>GSHMIKVLSPAKINLGLWVLGRLPSGYHEILTLYQEIPFYDEIYIREGVLRVETNIGIPQEENLVYKGLREFERITGIEINYSIFIQKNIPPGAGLGGGSSNLAVVLKKVNELLGSPLSEEELRELVGSISADAPFFLLGKSAIGRGKGEVLEPVETEISGKITLVIPQVSSSTGRVYSSLREEHFVTPEYAEEKIQRIISGEVEEIENVLGDIARELYPEINEVYRFVEYLGFKPFVSGSGSTVYFFGGASEELKKAAKMRGWKVVELEL[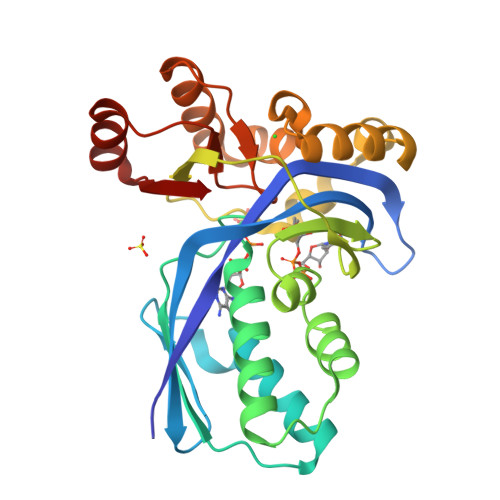2x]> SSDRPRGRDPVNPEKLLVITVATAETEGYLRFLRSAEFFNYTVRTLGLGEEWRGGDVARTVGGGQKVRWLKKEMEKYADREDMIIMFVDSYDVILAGSPTELLKKFVQSGSRLLFSAESFCWPEWGLAEQYPEVGTGKRFLNSGGFIGFATTIHQIVRQWKYKDDDDDQLFYTRLYLDPGLREKLSLNLDHKSRIFQNLN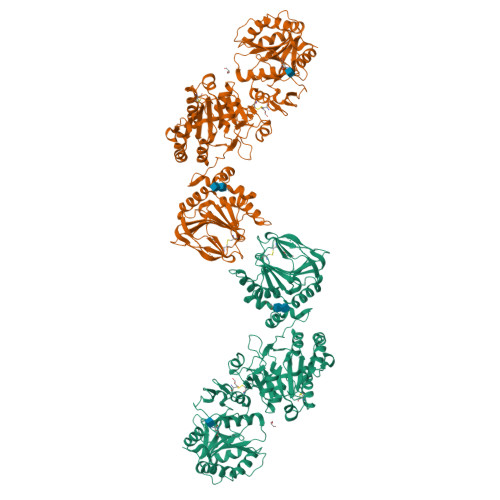GALDEVVLKFDRNRVRIRNVAYDTLPIVVHGNGPTKLQLNYLGNYVPNGWTPEGGCGFCNQDRRTLPGGQPPPRVFLAVFVEQPTPFLPRFLQRLLLLDYPPDRVTLFLHNNEVFHEPHIADSWPQLQDHFSAVKLVGPEEALSPGEARDMAMDLCRQDPECEFYFSLDADAVLTNLQTLRILIEENRKVIAPMLSRHGKLWSNFWGALSPDEYYARSEDYVELVQRKRVGVWNVPYISQAYVIRGDTLRMELPQRDVFSGSDTDPDMAFCKSFRDKGIFLHLSNQHEFGRLLATSRYDTEHLHPDLWQIFDNPVDWKEQYIHENYSRALEGEGIVEQPCPDVYWFPLLSEQMCDELVAEMEHYGQWSGGRHEDSRLAGGYENVPTVDIHMKQVGYEDQWLQLLRTYVGPMTESLFPGYHTKARAVMNFVVRYRPDEQPSLRPHHDSSTFTLNVALNHKGLDYEGGGCRFLRYDCVISSPRKGWALLHPGRLTHYHEGLPTTWGTRYIMVSFVDPAAA The THDI mediates binding of Myo3 to its cargo protein Espin1 (Ectoplasmic specialization protein 1) and allows Myo3 to transport Espin1 to the tips of actin bundle-based structures such as filopodia and stereocilia. Espin1 is the longest isoform in the family and contains a stretch of ankyrin repeats (AR) in its N-terminus. Here, we discover that both Myo3a and Myo3b contain two highly similar repeat sequences in their THDI region, each capable of independently binding to Espin1-AR with high affinity. The high resolution crystal structures of each of the two binding sequences from Myo3b in complex with Espin1-AR not only reveal the molecular basis governing the specific interaction between Myo3 and Espin1, but also allow us to discern the Myo3-mediated release of the auto-inhibition mechanism of Espin1.

We have also determined the Espin1-AR/Myo3b-ARB2 complex at a resolution of 2.3 Å. The structure of the complex and the binding mode of Myo3b-ARB2 to Espin1-AR are highly similar to what are observed in the Espin1-AR/Myo3b-ARB1 complex, directly confirming our earlier conclusion that the two repeat sequences in Myo3-THDI bind to Espin1-AR with similar binding mode and affinity. Comparing the structures of Espin1-AR in complex with Myo3b-ARB1 and Myo3b-ARB2, the ‘YY’ motif and the ‘KxL’ motif are essentially in the same places. Despite the high similarity, there are still a few minor differences. First of all, the C-terminal α-helix of ARB2 is shorter. The interaction is mediated by a hydrogen bond between Asp1294 and Tyr144, instead of the more extensive interaction observed in Myo3b-ARB1 complex. Moreover, the positively charged residues in the N-terminus of ARB2 cannot be reliably built, probably due to the high salt concentration in the crystallization buffer (1.6 M ammonium sulfate). Nonetheless, clear electron density can be observed near the negatively charged surface. Indeed, substitutions of these positively charged residues with Ala weakened the binding. Furthermore, the involvement of more positively charged residues of ARB2 may compensate for the less extensive interaction in its shorter C-terminal helix, thus resulting in a similar binding affinity to Espin1-AR as ARB1 does (107 nM for ARB1 vs 53 nM for ARB2, Figure 1C2 and C3).

>GSMALEQALQAARRGDLDVLRSLHAAGLLGPSLRDSLDALPVHHAARSGKLHCLRYLVEEVALPAVSRARNGATPAHDAAATGYLSCLQWLLTQGGCRVQEKDNSGATVLHLAARFGHPDVVKWLLYQGGANSAITTDTGALPIHYAAAKGDLPSLKLLVGHYPEGVNAQTNNGATPLYLACQEGHLEVTKYLVQECSADPHLRAQDGMTPLHAAAQMGHNPVLVWLVSFADVSFSEQDHDGATAMHFAASRGHTKVLSWLLLHGAEISQDLWGGTPLHDAAENGELECCQILAVNGAGLDVRDHDGYTAADLAEFNGHTHCSRYLRTVQTLSLEHRVLSRDQSMDLEAKQLDS[2x];>SQRKPRKLGQIKVLDGEDQYYKCLSPGACAPEETHSVHPFFFSSSPREDPFAQH[2x]> MRGSHHHHHHGMASLNRESSNRAKIPEIK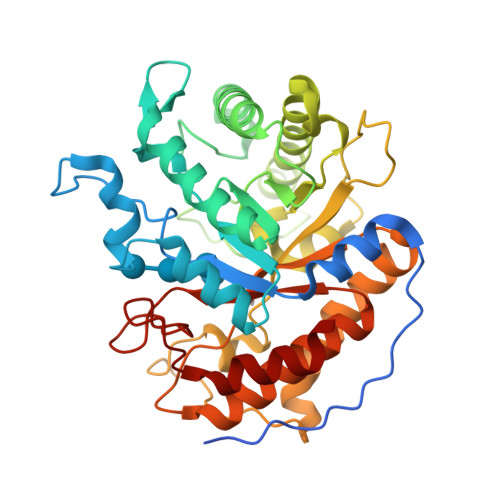IASRKIPNNAALKFVKDMKIGWNLGNTFDAAFENPSFDDELLYETAWCGVKTTKQMIDTVKKAGFNTIRIPVSWHNHVTGSNFTISKRWLDRVQQVVDYAMKNKMYVIINIHHDIMPGYYYPNSQHLQTSIKYVKSIWTQVATRFKNYNDHLIFEAVNQPRLTGSRFEWWLDMNNPECRDAVEAINKLNQVFVDTVRSTGGNNVSRYLMVPGYAAAPEYVLIDEFKIPKDSSKYKNRIIISVHAYRPYNFALQAPNESGSVSEWSVNSEESRRDIDYFMDKLYDKFVSKGIPVVIGEFGARDKNGNLQSRVEFAAYYVRAARARGITCCWWDNNAFYGNGENFGLLDRKTLKWVYPEIVSAMMKYAR>MPELEVKGKKLRLDEDGFLQDWEEWDEEVAEALAKDTRFSPQPIELTEEHWKIIRYLRDYFIKYGVAPPVRMLVKHCKKEVR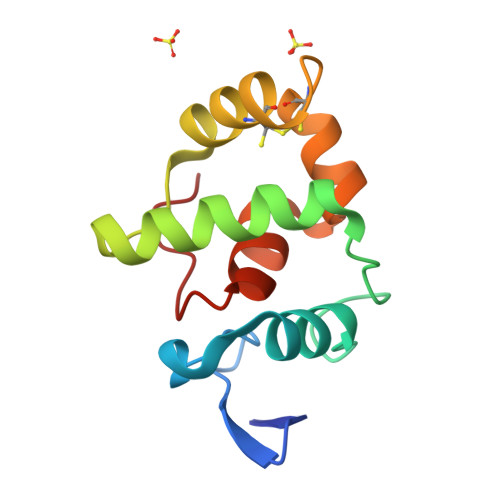PDCNLQYIYKLFPQGPAKDACRIAGLPKPTGCV[3x]> MRLGMVIDLQKCVGCGGCSLACKTENNTNDGIHWSHHIATTEGTFPDVKYTYIPTLCNHCDDAPCVKVCPTGAMHKDKRGLTLQNNDECIGCKKCMNACPYGVIS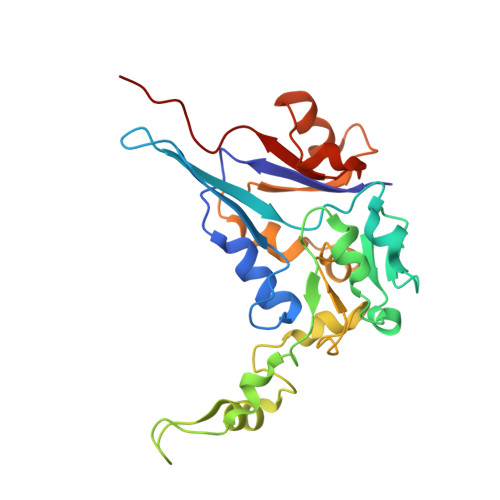FNAATPHRRWQDDSEVVANGTVSPLMLLKRTGATATPNENPERGDTYPMIRPKRTTEKCTFCDHRLDKGLNPACVDACPSEARVIGDLDDPQSKVSQLIKLHKPMQLKPEAGTGPRVFYIRSFGVKTAY>MGSITENTSWNKEFSAEAVNGVFVLCKSSSKSCATNDLARASKEYLPASTFKIPNAIIGLETGVIKNEHQVFKWDGKPRAMKQWERDLTLRGAIQVSAVPVFQQIAREVGEVRMQKYLKKFSYGNQNISGGIDKFALEGQLRISAVNQVEFLESLYLNKLSASKENQLIVKEALVTEAAPEYLVHSKTGFSGVGTESNPGVAWWV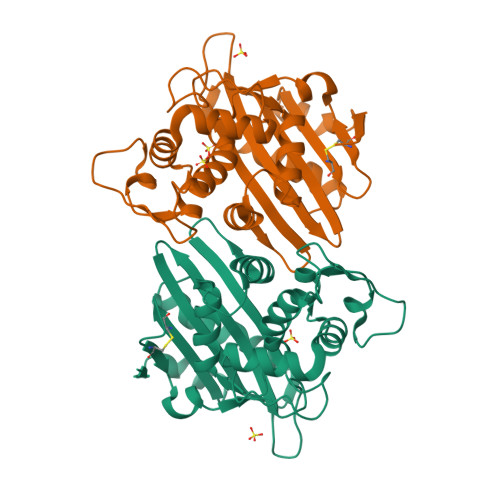GWVEKETEVYFFAFNMDIDNESKLPLRKSIPTKIMESEGIIGG[2x]> GCAUUGG;> CC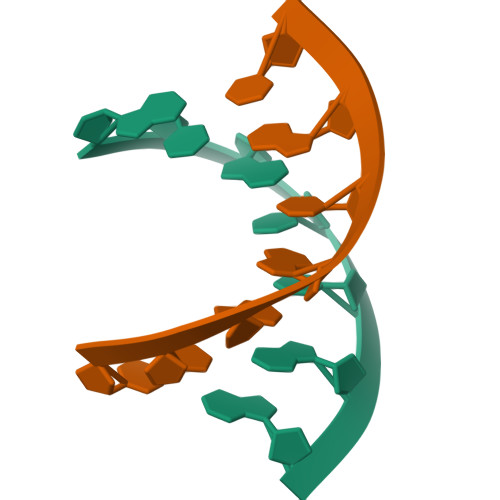AAUGC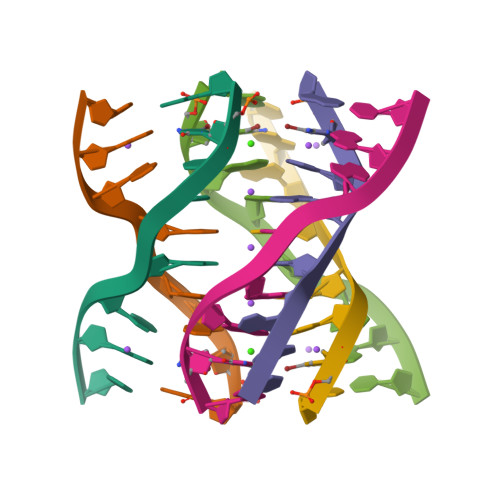>[2x]GCGGGAGC5'-O-[(S)-ethoxy(hydroxy)phosphoryl]adenosine | C12 H18 N5 O7 P | 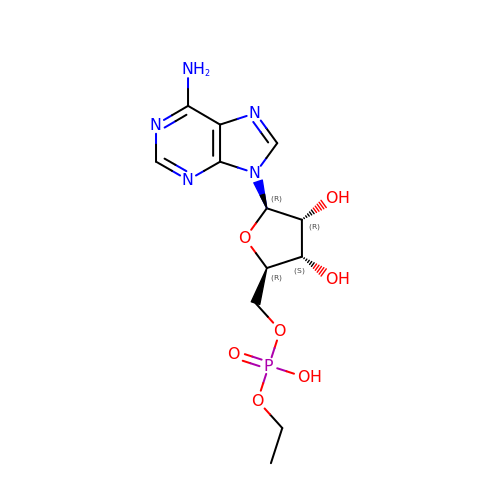MXYRBUKSSSUFQO-WOUKDFQISA-N> IVGGQECKDGECPWQALLINEENEGFCGGTILSEFYILTAAHCLYQAKRFKVRVGDRNTEQEEGGEAVHEVEVVIKHNRFTKETYDFDIAVLR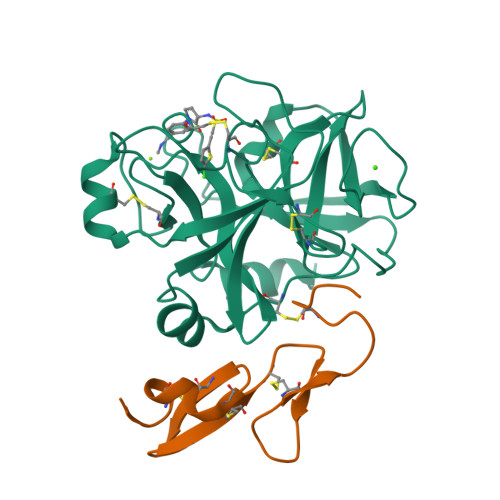LKTPITFRMNVAPACLPERDWAESTLMTQKTGIVSGFGRTHEKGRQSTRLKMLEVPYVDRNSCKLSSSFIITQNMFCAGYDTKQEDACQGDSGGPHVTRFKDTYFVTGIVSWGEGCARKGKYGIYTKVTAFLKWIDRSMKTRGLPKAKSHAPEVITSSPLK;> EEMKKGHLERECMEETCSYEEAREVFEDSDKTNEFWNKYKDGDQCETSPCQNQGKCKDGLGEYTCTCLEGFEGKNCELFTRKLCSLDNGDCDQFCHEEQNSVVCSCARGYTLADNGKACIPTGPYPCGKQTLER>MSGTEEAILGGRDSHPAAGGGSVLCFGQCQYTAEEYQAIQKALRQRLGPEYISSRMAGGGQKVCYIEGHRVINLANEMFGYNGWAHSITQQNVDFVDLNNGKFYVGVCAFVRVQLKDGSYHEDVGYGVSE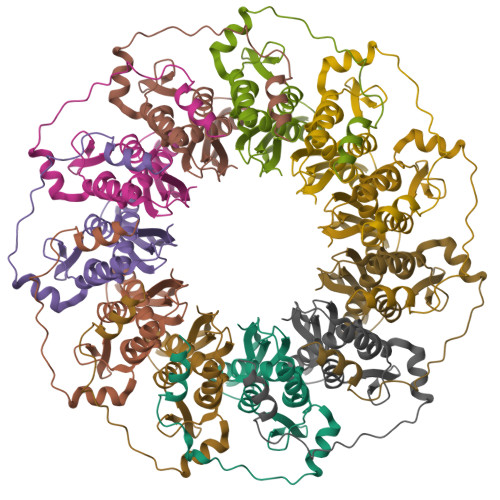GLKSKALSLEKARKEAVTDGLKRALRSFGNALGNCILDKDYLRSLNKLPRQLPLEVDLTKAKRQDLEPSVEEARYNSCRPNM[11x]>AMADLEQKVLEMEASTYDGVFIWKISDFARKRQEAVAGRIPAIFSPAFYTSRYGYKMCLRIYLNGDGTGRGTHLSLFFVVMKGPNDALLRWPFNQKVTLMLLDQNNREHVIDAFRPDVTS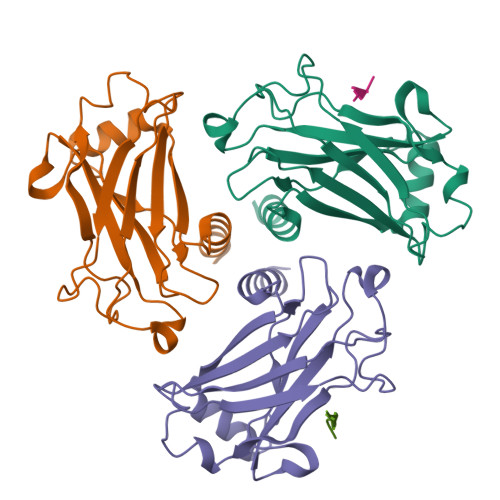SSFQRPVNDMNIASGCPLFCPVSKMEAKNSYVRDDAIFIKAIVDLTGL[6x];>[5x]XGAAQEE Periplasmic adaptor proteins are essential components of bacterial tripartite multidrug efflux pumps. BesA shows the archetypal linear, flexible, multi-domain architecture evident among proteobacteria and retains the lipoyl, β-barrel and membrane-proximal domains that interact with the periplasmic domains of the inner membrane transporter. However, it lacks the α-hairpin domain shown to establish extensive coiled-coil interactions with the periplasmic entrance helices of the outer membrane-anchored TolC exit duct. The adaptor multidomain structure is conserved throughout proteobacteria, but primary sequence comparison in the spirochete Borrelia burgdorferi suggested that a tripartite MDR pump, BesABC, included an adaptor that appeared to lack an α-hairpin.

The crystal structure of the complete BesA protein was solved by SAD in three space groups, P212121 (2.35 Å resolution), P21 (2.5 Å) and C2 (2.6 Å), in which either a monomer (C2) or four intertwined head-to-tail monomers (P21 and P212121) are present in the asymmetric unit. The BesA monomer shows the archetypal, multidomain adaptor topology, with the MP, β-barrel, and lipoyl domains in linear arrangement (coloured orange, yellow and green, respectively). However, the expected final α-hairpin domain is completely absent, confirming what was predicted from sequence analysis, leaving only a nine residue loop (Pro106 to Leu114, blue in Fig. 1B) linking the two halves of the lipoyl domain. Density for this loop is visible only in the C2 monomer where it is stabilised by the loop of a neighbouring monomer in the crystal lattice, but high B-factors here and poorly defined density for the P212121 or P21 monomers indicate the small loop is highly flexible. In both the data-based assembly model of AcrAB-TolC and the in vitro co-crystal structure of an adaptor-transporter (CusBA) subcomplex tripartite pump assembly is facilitated by the flexibility of the adaptor’s serially-linked domains, which was confirmed by MD analysis of the closely related MexA. This ‘hinge’ flexibility at the inter-domain linkers is also evident in the BesA variant space groups which show movement of the lipoyl domain, relative to the other domains.

> GSHMVGDNKLDDKNIDKEKESSYRFPVIAMKVKKGILSDYLSLNGDVDTKVKADIFPDAVGKITSLRIKLGAYVQKGQIVATLDPSRPGSVYLKSPVRAPISGYILNITKKIGETVNPQSNIAVVGRIDTKQILTYVSEKYISNIKVGNDAIIEVGAYSNEKFKAKVSEISPILDSKSRTIEVYLTPIGSNLDKLIIGMFSKIKLITKRFKDVIKISREAVVEREGKKFVFKVDLESKSVQMLPITVLFEIDNIVALSGEVEENDLIVVEGMSALSNGSLINLVDTKEGLSAESNI> HMYELTEDFKLRKITKYELDGVDEREDLLVIPPSSKAGPCGNGCLFCYLLQNPPEMIYRVARHDTLNDPTLEERIRYARKHYDLWIRVTDTSGNVKFDENRIKSLYEAGLDEIQISVHTTKKDVRIKLMRNRHAGKLIDLLPLVAKHFRTIADIILTPGFNVDDIGEIIEDLDSMGVHEVRLFPVGVTKYNRFEIRPLTKEELSYVKEVALEKDKELGIKVVIPPIFLALLGEFTTGLEPFNIEPEFPTYIFTGELAYPEMKRLFPRIKVVMVKNEFFGGNIGTAGLLTGRDVLREVERLPEVDFGLILLPELMFYGDMTLDGWRRQDLFSKILIEKGYIVETALEPTEIPKVIEKIS

Cobalamin (Cbl)-dependent radical S-adenosylmethionine (SAM) enzymes constitute a large subclass of radical SAM (RS) enzymes that use Cbl to catalyze various types of reactions, the most common of which are methylations. Bioinformatic analysis of Mmp10 identified DUF512 (Domain of Unknown Function 512) as a potential Cbl-binding domain in RS enzymes. X-ray crystal structures of DUF512-containing proteins from Clostridium sporogenes and Pyrococcus furiosus show unique architectural features and confirm the presence of a C-terminal Cbl-binding domain like that of Mmp10. We have uncovered the “Unknown Function” of the DUF512 protein domain, which is to bind the biological cofactor Cbl.

pfDUF512 belongs to a subset of DUF512-containing proteins that do not contain PDZ domains. pfDUF512 was crystallized under anoxic conditions in the presence of SAH, and its structure was determined to a resolution of 2.07 Å. The enzyme contains an N-terminal RS domain (residues 1–222) and a C-terminal Cbl-binding domain (residues 223–357) (topology diagram in Figure S5B). The RS domain has an antiparallel β-sheet (residues 1–14) followed by a loop (L1, residues 15–24) that connects to the TIM barrel core. Although pfDUF512’s substrate is unknown, in the current structure, L1 seems to close the active site of pfDUF512 by forming stabilizing interactions with the acetamide and DMB tail moieties of Cbl. The RS domain of pfDUF512 has a unique (βα)5 TIM barrel core, with the FeS cluster ligated by Cys39, Cys43, and Cys46. A molecule of 5′-dA is observed above the cobalt ion of cobalamin. The ligand (SAH) in the active site binds in an unusual position, neither ligated to the unique iron of the cluster, as seen in Mmp10, nor close to Cbl, as observed in csDUF512. SAH’s ribosyl and methionyl moieties have poor electron density, with very few hydrogen-bonding interactions. By contrast, there is significant electron density for the adenine portion of SAH, which binds approximately in the same position, maintaining a similar hydrogen-bonding network, as observed for Mmp10 and csDUF512. We hypothesize that the presence of 5′-dA above Cbl interferes with the SAH/SAM binding pocket and disrupts the binding of SAH.>[8x]HTLSTLAALPAAEIVRLA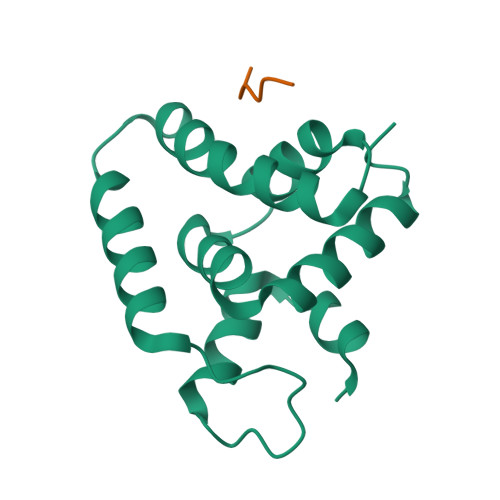NSQSSSGLPLPKADPATVKATDDFIDSLQGKAAHDQKQKLGDQLFKKIRTFGVKGAPKLTIHLLDSEDLRALAHLMNSYEDVLKEKVQHKVAAGLNKVKGAPKLTIHLLDSEDLR;>[8x]DEFIYP>[2x]MKTLLKNSLTFLLMLMPVLAFAQQAPQIMNVSARQTTSLDG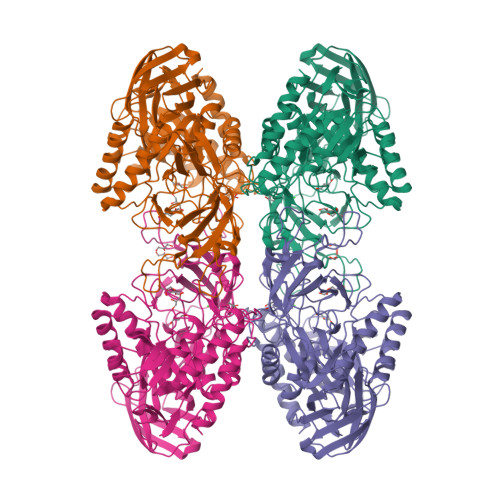QWKTIVDPFENGYYDYRLKPYDGGYAQDKTYSDKTKLQEYDFETDKLLFVPGDWNTQRPQLYYYEGTVWYRKHFEYSLQPGKRLFLNFGAVNYEAIVWLNGKRLGRHIGGFTPFNFEITNLLKEGTNSLVVKVDNKRLPEAVPTVNADWWNFGGITRPVTLIEMPATYIRDYYVQLAKDDKNMIEGWVQLEGSDKEQKITLDIPELKVKKEVTTDANGYASFLIKSKPILWTPENPKLYAVNLASETDKVSDEIGFRTIRTEGIKILLNDKEIFCRGISIHEETPYYSGRAYSKDHAHTLLSWAKELGCNFVRLAHYPHNEEMVREAERMGFLVWSEIPVYWTIHWENKDTYQNAEQQLCDMIARDKNRCNIIIWSIANETPHSKTRLTFLSNLANKARSLDSVRLIGAAMEKEEVQPGVLTVNDPLGELLDIISFNEYVGWYDGDSEKCDRVNWTFDTQKPVFISELGGGALYGHHGSPKERFTEEYQEDLYIRHVNMLKRIPGLAGTTPWILKDFRSPRRHVPEIQDDFNRKGLVSDKGQKKKAFFVLQKWYKELTEAYK> AIVSSVDRKIFVLLRDGRMLFGVLRTFDQYANLILQDCVERIYFSEENKYAEEDRGIFMIRGENVVMLGEVDIDKEDQPLEAMERIPFKEAWLTKQKNDEK;> SENLYFQGSGSLFFSFFKTLVDQEVVVELKNDIEIKGTLQSVDQFLNLKLDNISCTDEKKYPHLGSVRNIFIRGSTVRYVYLNKNMVDTNLLQDATRREVMTERK;> METPLDLLKLNLDERVYIKLRGARTLVGTLQAFDSHCNIVLSDAVETIYQLNNEELSESERRCEMVFIRGDTVTLISTPSEDDDGAVEI;> MLPLYLLTNAKGQQMQIELKNGEIIQGILTNVDNWMNLTLSNVTEYSEESAINSEDNAESSKAVKLNEIYIRGTFIKFIKLQDNIIDKVKQQINSNNNSNSNGPGHKRYYNNRD;> MSLPEILPLEVIDKTINQKVLIVLQSNREFEGTLVGFDDFVNVILEDAVEWLIDPEDESRNEKVMQHHGRMLLSGNNIAILVPGGKKTPTEAL;> MSGKASTEGSVTTEFLSDIIGKTVNVKLASGLLYSGRLESIDGFMNVALSSATEHYESNNNKLLNKFNSDVFLRGTQVMYISEQKI;> MHQQHSKSENKPQQQRKKFEGPKREAILDLAKYKDSKIRVKLMGGKLVIGVLKGYDQLMNLVLDDTVEYMSNPDDENNTELISKNARKLGLTVIRGTILVSLSSAEGSDVLYMQK;> SSYAFNNGNGATNLNKSGGKKFILELIETVYEEILDLEANLRNGQQTDSTAMWEALHIDDSSYDVNPFISMLSFDKGIKIMPRIFNFLDKQQKLKILQKIFNELSHLQIIILSSYKTTPKPTLTQLKKVDLFQMIILKIIVSFLSNNSNFIEIMGLLLQLIRNNNVSFLTTSKIGLNLITILISRAALIKQDSSRSNILSSPEISTWNEIYDKLFTSLESKIQLIFPPREYNDHIMRLQNDKFMDEAYIWQFLASLALSGKLNHQRIIIDEVR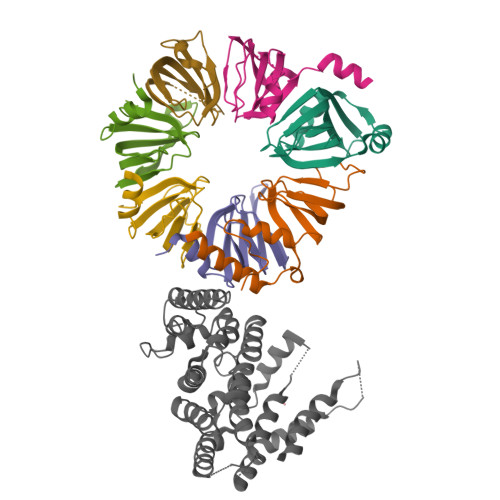DEIFATINEAETLQKKEKELSVLPQRSQELDTELKSIIYNKEKLYQDLNLFLNVM> MFAGRLMVRSIVGRACLATMGRWSKPQAHASQV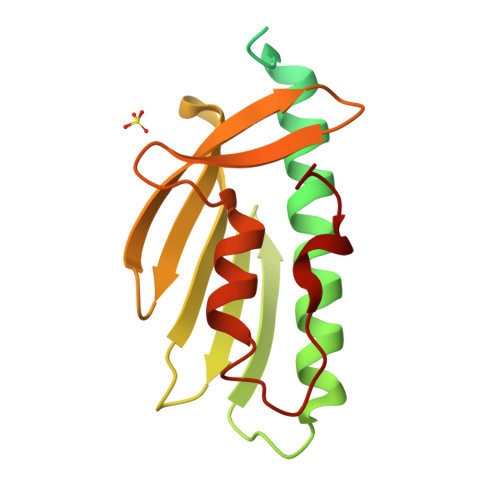ILPSTPAIAAVAIQCEEFTANRRLFSSQIETESTLDGATYERVCSDTLDALCDYFEELTENASELQGTDVAYSDGVLTVNLGGQHGTYVINRQTPNKQIWLSSPTSGPKRYDFVGTVAAGRWIYKHSGQSLHELLQQEIPGILKSQSVDFLRLPYCS>MTMITHHHHHHGSNSYYTEENHGPFELINIGPLPLEEGRCMPECLLAVAVHGALNADKSNAILVPTWYSGTSKAMEQIYIGEGRALDPSKYCIIVVNQIGNGLSSSASNTGGSLAGPGFANVRIGDDVSAQHTLLTEYFGIESLALVVGGSMGAQQTYEWAVRYPDFVKRAAAIAGTARNSEHDFLFTEILIEAITTDPAFQAGLYRSSSAVAAGLERHAKLWTLMGWSPEFFRTGRHKALGFESMQMFVDGFMKRYFAPMDPNNLLTMAWKWQRGDVS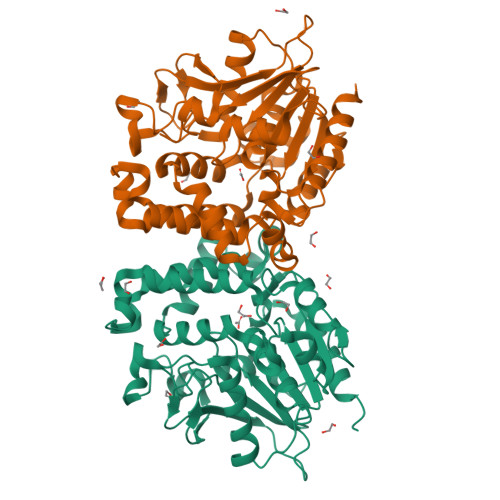RHTGGDLAKALGRIKAKTYVMPISHDQFFTVDDCLSEQKMIPNSEFRPLRSIDGHLGLFGTDAQMLDQLDAHLAELLSSPAY[6x]>[3x]MRGSHHHHHHGSLVPRGSMKKVSVIMPTFNNGEKLHRTISSVLNQTMKSTDYELIIIDDHSNDNGETLNVIKKYKGLVRFKQLKKNSG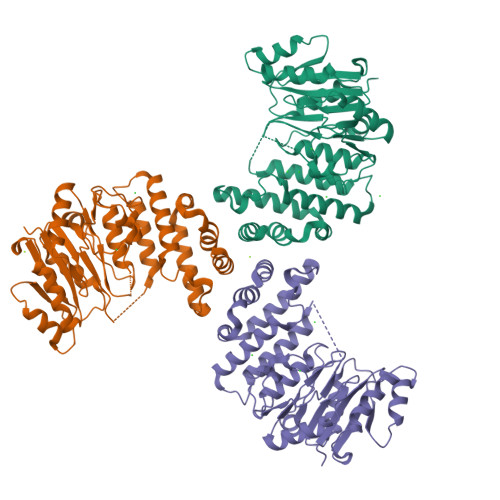NASVPRNTGLKMSKAEYVFFLDSDDLLHERALEDLYNYGKENNSDLIIGKYGVEGKGRSVPKAIFEKGNVAKADIIDNSIFYALSVLKMFKKSVIDKNKIKFKTFSKTAEDQLFTIEFLMNSKNYSIKTDYEYYIVVNDFESSNHLSVNKSTGNQYFATINEIYKAIYKSPIYKNQEKRHQLAGKYTTRLLRHGQKKNFANSKMKYEDKIEWLNNFSKTINKVPRDSDKYVTQIFNLKLEAIRQNDLLAVMIADKLL> TIGSEFQNDIPDLYSVFKDYFPIGVAVDPSRLNDTDPHAQLTAKHFNMLTAENAMKPESLEPEEGRYNFEDADRIVAFAEKHGMKMRGHTLVWHQQVPDWFFLDENGNPMVDETDPKNREANREELRQRMENHIKTVAGRYKGKIYAWDVVNEVFNDDGTLRNSAWYQIIGPDYIEEALRAAHEADPNAKLFINDYNIENWSHAKTQAMYNMVRDFKERGVPVDGVGMQGHISLYYPSLEEIEKALKAFAALGVEIMITELDVNTQGDVSPDALQEQAERMRDLFELFKKHSDKITGVTFWGVADDQSWKNNFPVPGRTNAPLLFDRNYQPKPAFWAIV

GH10 enzymes hydrolyze the β-1,4 glycosidic bonds linking the xyloside units that comprise the backbone of the polysaccharide xylan, which is second only to cellulose in abundance in the plant cell wall; xylanases are, therefore, essential for biomass degradation. The design method is inspired by the evolution of new enzymes in nature through recombination, insertion, deletion, and mutation. It starts by computationally segmenting all structures belonging to a modular enzyme family along structurally conserved sites and assembling the resulting modular fragments to generate a huge combinatorial diversity of backbones. Instead of using the natural sequences of the fragments, as in natural evolution or laboratory genetic recombination, we next design the sequence of the entire protein (>300 amino acids) to maximize compatibility between the fragments and stabilize the active-site geometry.

We then selected the eight most active designs and two natural GH10 enzymes for quantitative kinetic analysis with the chromogenic substrate 4-nitrophenyl β-xylobioside (O-PNPX2). The active designs spanned five orders of magnitude in catalytic efficiency. For instance, the most active GH10 design xyl3.1 and the least active one xyl8.3 exhibited OPNPX2 hydrolysis efficiencies of 9417 and 0.61 M-1 s-1, respectively. To understand what were the underlying structural reasons for this vast difference in efficiency, we determined their crystallographic structures. In both structures, the two catalytic Glu residues were positioned as in the design conception (<0.5 Å all-atom root-mean-square deviation (rmsd)). The high-activity design xyl3.1 was also atomically accurate throughout 13 active-site residues that form an intricate hydrogen-bond network surrounding the two catalytic Glu residues (<1 Å all-atom rmsd), and indeed, across the entire protein, with a total backbone rmsd of 0.7 Å. Furthermore, missing electron density in β-α loops 7 and 8 suggested that at least parts of the active-site pocket were mobile, although design accuracy was high throughout the segments of the design model and experimental structure that could be aligned (0.9 Å backbone rmsd). We, therefore, concluded that accurate positioning of the two catalytic Glu residues was crucial to obtain any level of activity, and that high levels of activity depended on atomic precision and preorganization in a large network of polar residues that surround the catalytic residues.(~{Z})-4-formamido-4-oxidanylidene-but-2-enoic 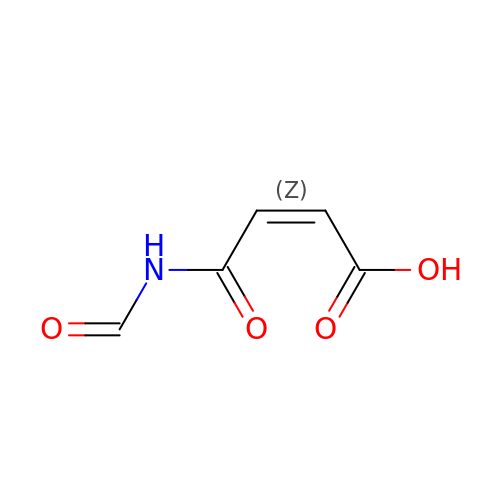acid | C5 H5 N O4 | HSKSAKBZUITULZ-UPHRSURJSA-N>[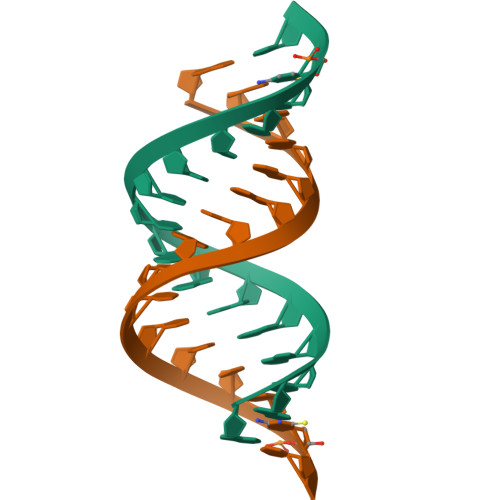2x]AGAGAAGAUCUUCUCU BEST1-4 proteins are expressed in the plasma membrane and form Ca2+-activated Cl- channels by assembling as pentamers. The channel comprises five BEST1 subunits arranged symmetrically around a central ion pore that is ~95 Å long. The diameter of the pore varies along its length and contains two constrictions, the ‘neck’ and the ‘aperture’, both of which are lined by hydrophobic amino acids. To address these questions we determined a series of cryo-electron microscopy (cryo-EM) structures of chicken BEST1 with and without Ca2+ in activated, deactivated, and inactivated states that represent the major gating transitions of the channel.

We find that the W287F mutation (BEST1345 W287F) produces channels with dramatically altered gating. Whilst BEST1345 W287F retained normal Cl- versus K+ selectivity, the W287F mutation constitutively activates the channel, making it nearly insensitive to the presence or absence of Ca2+. Approximately, 80% of the Cl- current level through BEST1345 W287F is maintained when Ca2+ was chelated with EGTA, whereas currents through wild type BEST1 drop to zero. To understand the molecular basis of this behavior, we determined cryo-EM structures of BEST1345 W287F in the presence and absence of Ca2+ at 2.7 Å and 3.0 Å resolutions, respectively (Figure 4—figure supplements 1 and 2). Remarkably, in the absence of Ca2+, and in spite of missing density for Ca2+ and a disordered Ca2+-clasp region, the neck also adopts an open conformation. Thus, in accord with the electrophysiological recordings, the W287F mutation decouples Ca2+ binding from the conformational changes in the neck that are observed for the wild type channel. Modeling of the W287F mutation on a closed conformation of the channel introduces a void behind the neck, which we hypothesize energetically disfavors the closed conformation.

>TVTYTNRVADARLGTFSQLLLQWKGSIYKLLYSEFLIFISLYFAISLVYRLILSESQRLMFEKLALYCNSYAELIPVSFVLGFYVSLVVSRWWAQYESIPWPDRIMNLVSCNVDGEDEYGRLLRRTLMRYSNLCSVLILRSVSTAVYKRFPSMEHVVRAGLMTPEEHKKFESLNSPHNKFWIPCVWFSNLAVKARNEGRIRDSVLLQGILNELNTLRSQCGRLYGYDWISIPLVYTQVVTVAVYSFFLACLIGRQFLDPEKAYPGHELDLFVPVFTFLQFFFYAGFLKVAEQLINPFGEDDDDFETNWLIDRNLQVSLMAVDEMHQDLPILEKDLYWNEPDPQEGEEF[5x]> MGSSHHHHHHSQDPRACLKCKYLTNDEICPICHSPTSENWIGLLIV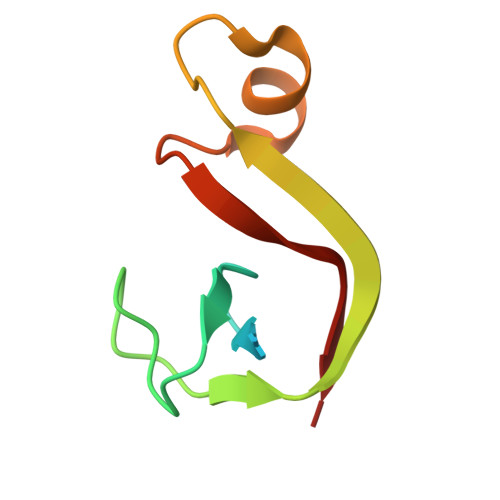INPEKSEIAKKAGIDIKGKYALSVKE>[2x]GSHMDSTTIQQNKDTLSQIVVFPTGNYDKNEANAMVNRLANIDGKYLNALKQNNLKIKLLSGKLTDEKEYAYLKGVVPKGWEGTGKTWDDVPG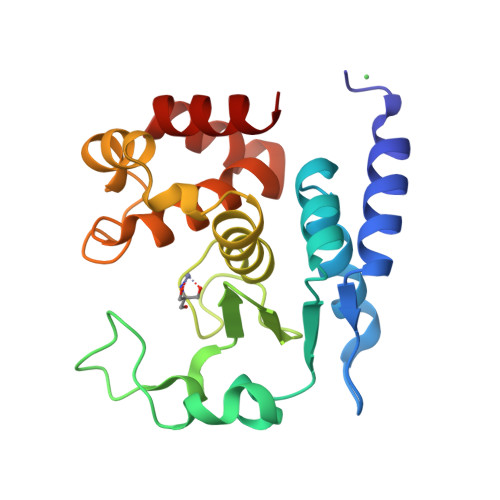LGGSTVALRIGFSNKGKGHDAINLELHETAHAIDHIVLNDISKSAQFKQIFAKEGRSLGNVNYLGVYPAEFFAESFAYYYLNQDTNSKLKSACPQTYSFLQNLAK> MAETESIDPEKLRDQLLDAFENKQNELKSSKAYYDAERRPDAIGLAVPLDMRKYLAHVGYPRTYVDAIAERQELEGFRIPSANGEEPESGGENDPASELWDWWQANNLDIEATLGHTDALIYGTAYITISMPDPEVDFDVDPEVPLIRVEPPTALYAEVDPRTRKVLYAIRAIYGADGNEIVSATLYLPDTTMTWLRAEGEWEAPTSTPHGLEMVPVIPISNRTRLSDLYGTSEISPELRSVTDAAAQILMNMQGTANLMAIPQRLIFGAKPEELGINAETGQRMFDAYMARILAFEGGEGAHAEQFSAAELRNFVDALDALDRKAASYSGLPPQYLSSSSD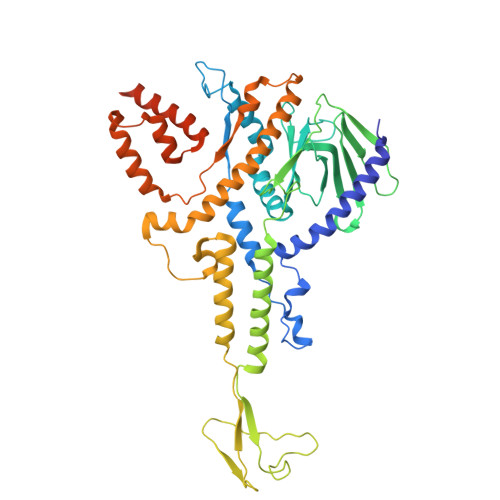NPASAEAIKAAESRLVKKVERKNKIFGGAWEQAMRLAYKMVKGGDIPTEYYRMETVWRDPSTPTYAAKADAAAKLFANGAGLIPRERGWVDMGYTIVEREQMRQWLEQDQKQGLGLIGSLYGASTPEGKPGEAPVGEPPAPEPDAA> NRRYDSEFQTMLQHLQPTAENAYEYFTKI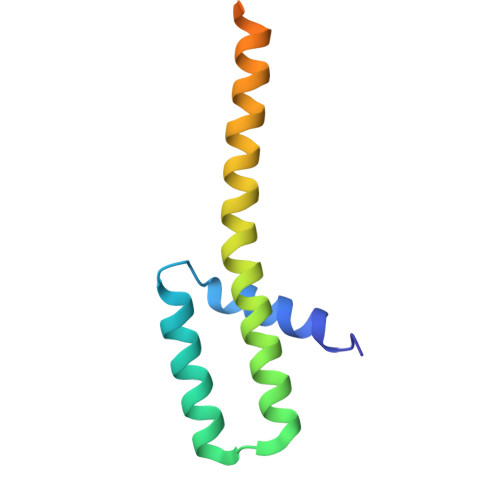ATSLFESGINWGRVVALLGFGYRLALHVYQHGLTGFLGQVTRFVVDFMLHHSIARWIAQRGGWVAALNLGNG>[2x]WDGKIDGTGTHAMIVTQGVSILENDLSKNEPESVRKNLEILKENMHELQLGSTYPDYDKNAYDLYQDHFWDPDTDNNFSKDNSWYLAYSIPDTGESQIRKFSALARYEWQRGNYKQATFYLGEAMHYFGDIDTPYHPANVTAVDSAGHVKFETFAEERKEQYKINTVGCKTNEDFYADILKNKDFNAWSKEYARGFAKTGKSIYYSHASMSHSWDDWDYAAKVTLANSQKGTAGYIYRFLHDVSEGNDPS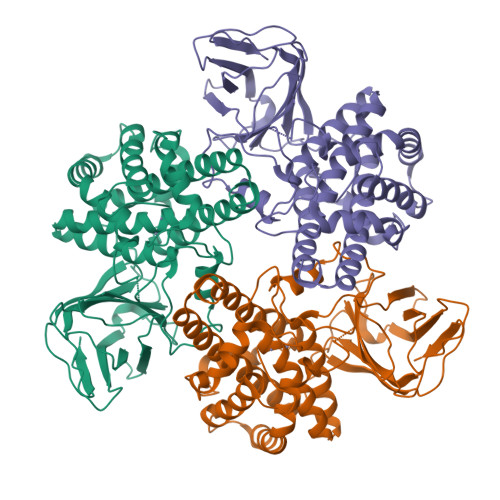VGKNVKELVAYISTSGEKDAGTDDYMYFGIKTKDGKTQEWEMDNPGNDFMTGSKDTYTFKLKDENLKIDDIQNMWIRKRKYTAFPDAYKPENIKVIANGKVVVDKDINEWISGNSTYNIK>MASSNLIKQLQERGLVAQVTDEEALAERLAQGPIALYCGFDPTADSLHLGHLVPLLCLKRFQQAGHKPVALVGGATGLIGDPSFKAAERKLNTEETVQEWVDKIRKQVAPFLDFDCGENSAIAANNYDWFGNMNVLTFLRDIGKHFSVNQMINKEAVKQRLNREDQGISFTEFSYNLLQGYDFACLNKQYGVVLQIGGSDQWGNITSGIDLTRRLHQNQVFGLTVPLITKADGTKFGKTEGGAVWLDPKKTSPYKFYQFWINTADADVYRFLKFFTFMSIEEINALEEEDKNSGKAPRAQYVLAEQVTRLVHGEEGLQAAKRITECLFSGSLSALSEADFEQLAQDGVPMVEMEKGADLMQALVDSELQPSRGQARKTIASNAITINGEKQSDPEYFFKEEERL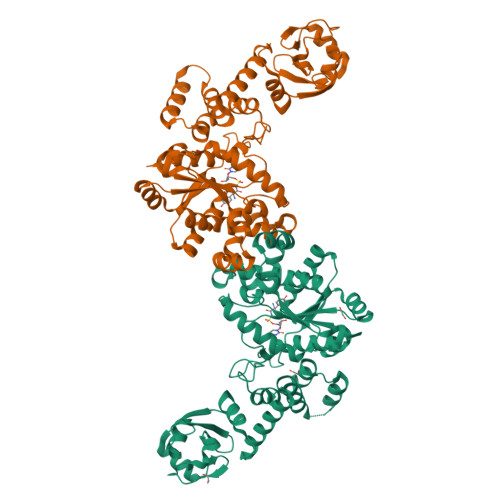FGRFTLLRRGKKNYCLICWK[2x]>MAEAASCARKGTKYAEGTQPFTVLIEGNIGSGKTTYLNHFEKYKNDICLLTEPVEKWRNVNGVNLLELMYKDPKKWAMPFQSYVTLTMLQSHTAPTNKKLKIMERSIFSARYCFVENMRRNGSLEQGMYNTLEEWYKFIEESIHVQADLIIYLRTSPEVAYERIRQ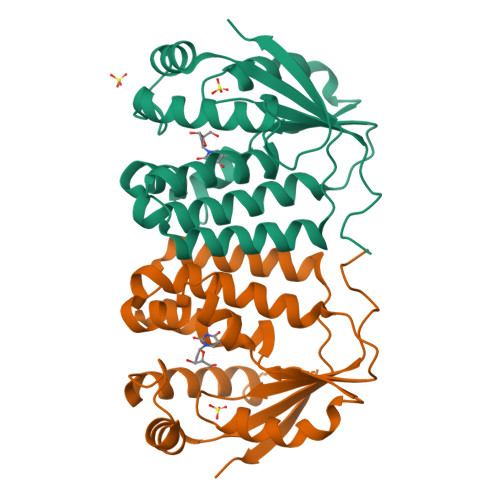RARSEESCVPLKYLQELHELHEDWLIHQRRPQSCKVLVLDADLNLENIGTEYQRSESSIFDAIS[8x]>RGSHHHHHHGSFTPSGTTGTTKLTVTEKCQVRVGDLTVAKT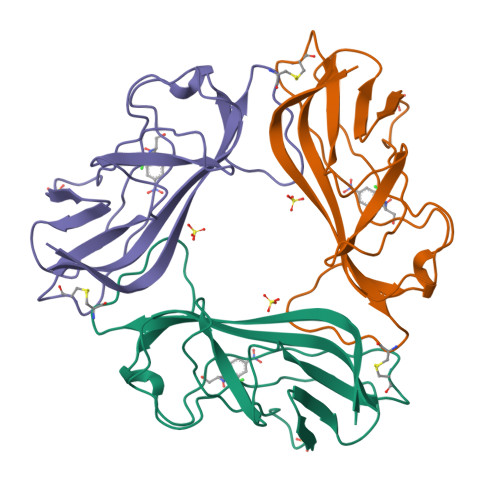RGQLTDAAPIGPVTVQALGCDARQVALKADTDNFEQGKFFLISDNNRDKLYVNIRPTDNSAWTTDNGVFYKNDVGSWGGIIGIYVDGQQTNTPPGNYTLTLTGGYWAK[6x]>[2x]MSENQEQEEVITVRVQDPRVQNEG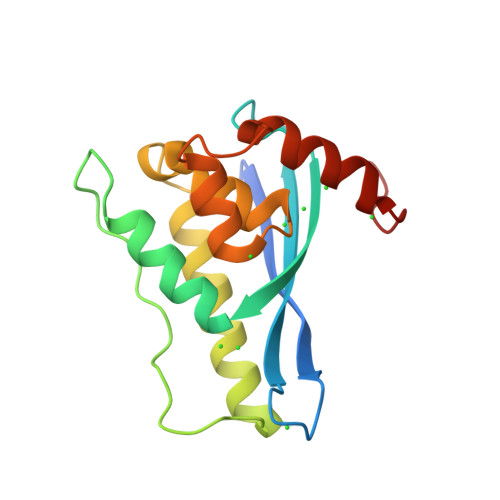SWNSYVDYKIFLHTNSKAFTAKTSCVRRRYREFVWLRKQLQRNAGLVPVPELPGKSTFFGTSDEFIEKRRQGLQHFLEKVLQSVVLLSDSQLHLFLQSQLSVPEIEACVSGQTKYSVEEAIHKFALMNLEHHHHHH>TSHHHHHMKKIEHKMVAVN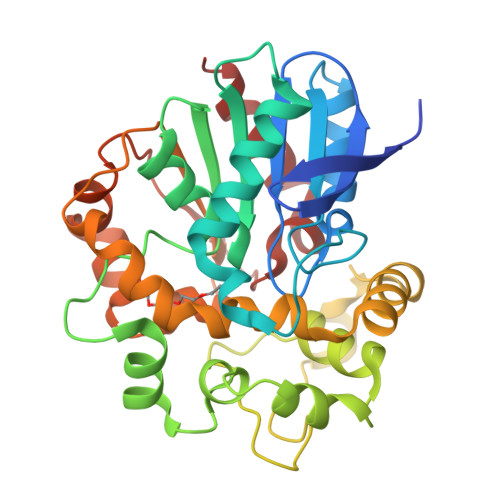GLNMHLAELGEGPTILFIHGFPELWYSWRHQMVYLAERGYRAVAPDLRGYGDTTGAPLNDPSKFSILHLVGDVVALLEAIAPNEEKVFVVAHDWGALIAWHLCLFRPDKVKALVNLSVHFSKRNPKMNVVEGLKAIFGEDHYISRFQVPGEIEAEFAPIGAKSVLKKILTYRDPAPFYFPKGKGLEAIPDAPVALSSWLSEEELDYYANKFEQTGFTGAVNYYRALPINWELTAPWTGAQVKVPTKFIVGEFDLVYHIPGAKEYIHNGGFKKDVPLLEEVVVLEGAAHFVSQERPHEISKHIYDFIQKF[2x]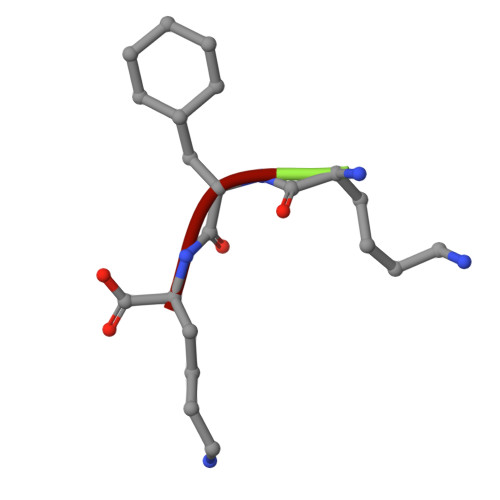> KAK>MKTINVFHYDAFTNKPNMGNPAGIVLDADGLTEEEMQRIAEKVGFNETSFVLSSEVADIRMRYFTPGYEMDLCGHGTVGTIYALRERGLLEEKASLTIETKAGILPIQIGVNENGETFIKMRQTAPQFKDFAGSKEELAHSIGLEVNDLDVSLPIVYGSTGNWTVIVPVKNLDVCERMKPNNEVFPSVLKEIPNASIHPICLETYDEKVHMHGRHFSSAYAGTIEDPVTGTASGVMGAYYATYVEKDFDHEMELIVEQGQEIHKDGRVTVYVTKDVESEKLQIDIAGTAVYVKEFEVLI[2x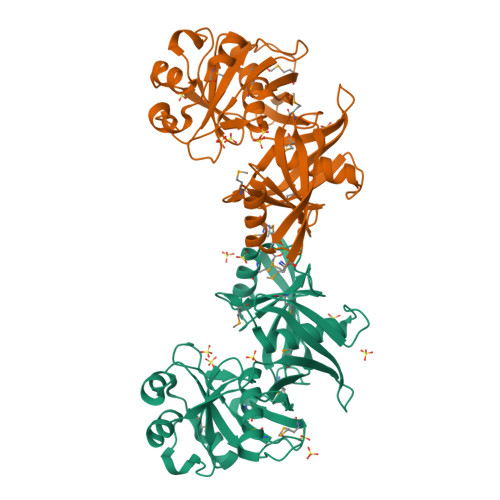]> MAQTVPYGIPLIKADKVQAQGFKGANVKVAVLDTGIQASHPDLNVVGGASFVAGEAYNTDGNGHGTHVAGTVAALDNTTGVLGVAPSVSLYAVKVLNSSGSGSYSGIVSGIEWATTNGMDVINMSLGGASGSTAMKQAVDNAYARGVVVVAAAGNSGNSGSTNTIGYPAKYDSVIAVGAVDSNSNRASFSSVGAELEVMAPGAGVYSTYPTNTYATLNGTSMASPHVAGAAALILSKH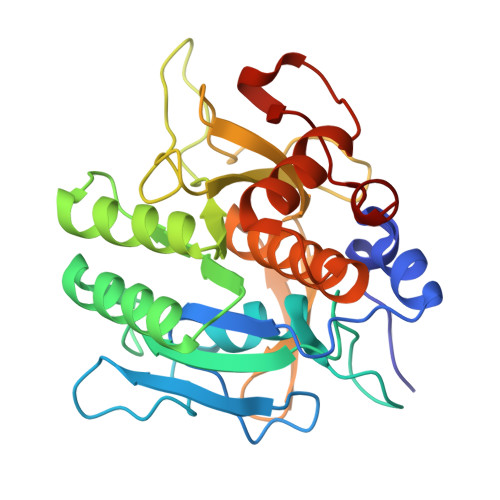PNLSASQVRNRLSSTATYLGSSFYYGKGLINVEAAAQ>[4x]MNIPLSGIIPPLVTPLLDDDVL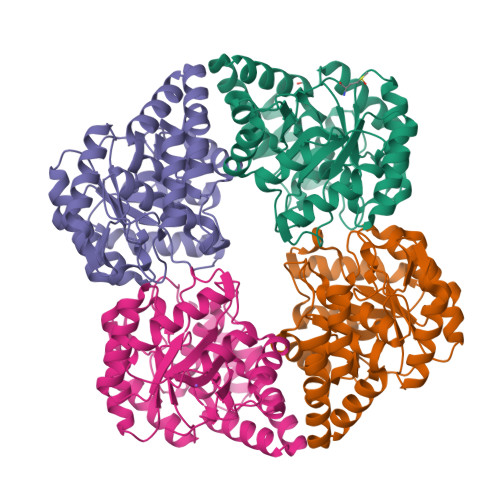DVEGLQRLIEHLIAGGVHALFVLGTTGESQSLSYKLRMEMIKNTCRIAKGRLPVLVCISDTSIVESVNLACLAADHGADAVVSAPPYYFATGQPELIEFYEHLLPQLPLPLFLYNMPTHTKVNFAPATIQRIAENPGVIGFKDSSANTVYFQSVMYAMKDNPDFSMLVGPEEIMAESVLLGAHGGVNGGANMFPELYVSLYNAAKNADMEEVRRLQEKVMQISATIYTVGQHGSSYLKGLKCALSLLGICSDYVAAPFHKFEQRERGKIWKALQNLGV>MGSDKIHHHHHHMKIDILDKGFVELVDVMGNDLSAVRAARVSFDMGLKD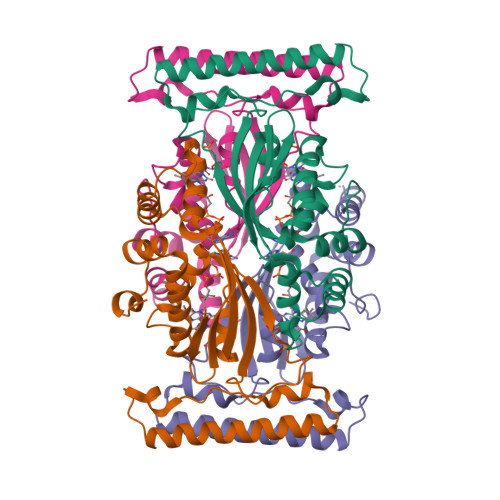EERDRHLIEYLMKHGHETPFEHIVFTFHVKAPIFVARQWFRHRIASYNELSGRYSKLSYEFYIPSPERLEGYKTTIPPERVTEKISEIVDKAYRTYLELIESGVPREVARIVLPLNLYTRAFATVNARSLMNFLNLRADSHAQWEIQQYALAIARIFKEKCPWTFEAFLKYAYKGDILKEVQV[4x]> MNLTIPFAKGHATENDFIIIPDEDARLDLTPEMVVTLCDRRAGIGADGILRVVKAADVEGSTVDPSLWFMDYRNADGSLAEMCGNGVRLFAHWLYSRGLVDNTSFDIGTRAGVRHVDILQADQHSAQVRVDMGIPDVTGLSTCDINGQVFAGLGVDMGNPHLACVVPGLSASALADMELRAPTFDQEFFPHGVNVEIVTELEDDAVSMRVWERGVGETRSCGTGTVAAACAALADAGLGEGTVKVCVPGGEVEVQIFDDGSTLTGPSAIIALGEVQIHHHHHH

DapF (EC 5.1.1.7), a pyridoxal 5-phosphate-independent amino acid racemase, catalyzes the stereochemical inversion between l,l-DAP and d,l-DAP. DapF plays an important role in the biosynthesis of l-lysine because DAP decarboxylase only recognizes d,l-DAP. Each CgDapF monomer consists of two distinct domains: an N-terminal domain (NTD; Met1–Asp131 & Gly268–Ile277) and a C-terminal domain (CTD; Met132–Thr267). Two catalytic cysteine residues are positioned at the active site, which is located at a cleft between the two domains.

To investigate the substrate binding mode of CgDapF, we determined the crystal structure of the protein in complex with the d,l-DAP product. In fact, although we added a mixture of the three DAP enantiomers (l,l-DAP, d,d-DAP, d,l-DAP) into the crystallization solution, we only observed density consistent with d,l-DAP in the electron density map. We suspect that the l,l-DAP substrate was converted to the d,l-DAP product during the crystallization procedure because we used the wild-type protein. The substrate binding site is located at a deep cleft formed between the two domains. It can be divided into two sub-sites, a catalytic sub-site and a recognition sub-site, where the d- and l-amino moieties of d,l-DAP are positioned, respectively. The two catalytic cysteine residues are located at the catalytic sub-site, and the amino group in the d-amino moiety is hydrogen bonded to the carboxyl group of Glu212. The carboxyl group of d,l-DAP on the side bearing the d-amino moiety, is stabilized through hydrogen bonds with the main chain nitrogen atoms of Gly84, Asn85, Gly222, and Thr223, and the side chains of Asn85 and Thr223. In the recognition sub-site, the carboxyl group of d,l-DAP on the side bearing the l-amino moiety is stabilized by direct interactions with the main chain of Arg213 and the side chains of Asn74, Asn159, Asn194, and Arg213. When we superimposed the apo-structure of CgDapF with that of the complex with d,l-DAP, it became evident that substrate binding had induced the CTD to move towards the NTD. In addition, the interactions between the reorganized CTD and the residues located at the entrance of the active site cleft result in a completely buried substrate binding site.>MAIAQLATEYVFSDFLLKEPTEPKFKGLRLELAVDKMVTCIAVGLPLLLISLAFAQEISIGTQISCFSPSSFSWRQAAFVDSYCWAAVQQKNSLQSESGNLPLWLHKFFPYILLLFAILLYLPPLFWRFAAAPHICSDLKFIMEELDKVYNRAIKAAKSARDLDMRDGACSVPGVTENLGQSLWEVSESHFKYPIVEQYLKTKKNSNNLIIKYISCRLLTLIIILLACIYLGYYFSLSSLSDEFVCSIKSGILRNDSTVPDQFQCKLIAVGIFQLLSVINLVVYVLLAPVVVYTLFVPFRQKTDVLKVY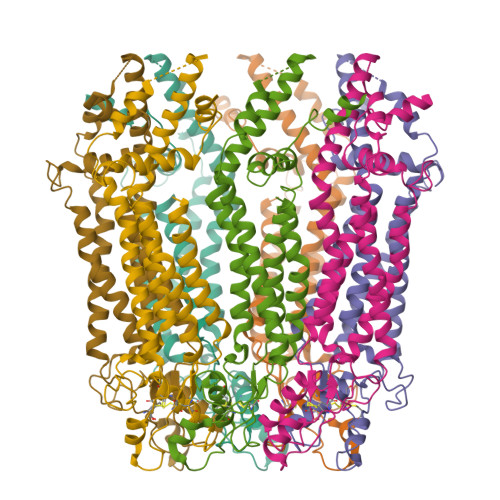EILPTFDVLHFKSEGYNDLSLYNLFLEENISEVKSYKCLKVLENIKSSGQGIDPMLLLTNLGMIKMDVVDGKTPMSAEMREEQGNQTAELQGMNIDSETKANNGEKNARQRLLDSSCGSGSHHHHHHHHHH[7x]>GEIRPTIGQQMETGDQRFGDLVFRQLAPNVWQHTSYLDMPGFGAVASNGLIVRDGGRVLVVDTAWTDDQTAQILNWIKQEINLPVALAVVTHAHQDKMGGMDALHAAGIATYANALSNQLAPQEGMVAAQHSLTFAANGWVEPATAPNFGPLKVFYPGPGHTSDNITVGIDGTDIAFGGCLIKDSKAKS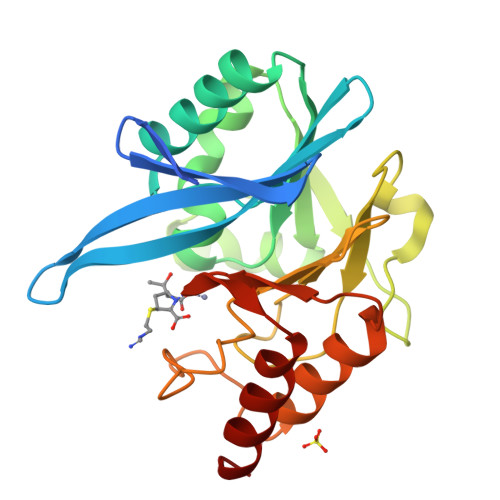LGNLGDADTEHYAASARAFGAAFPKASMIVMSHSAPDSRAAITHTARMADKLR[2x]> SLTFYPAWLTVSEGANATFTCSLSNWSEDLMLNWNRLSPSNQTEKQAAFSNGLSQPVQDARFQIIQLPNRHDFHMNILDTRRNDSGIYLCGAISLHPKLKIEESPGAE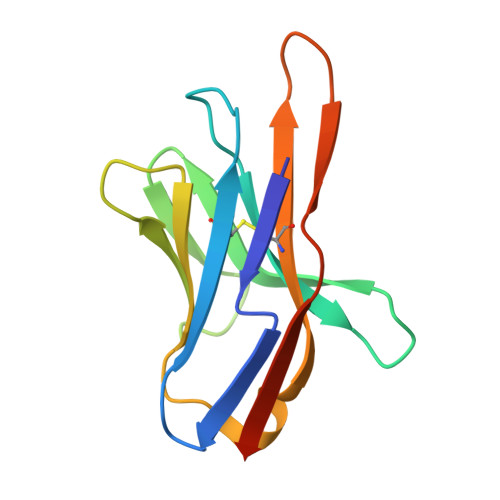LVVTERILE>MGSSHHHHHHSGAPGVDVDSSNDRAWRQTQLKVAELLIERQPEVAVGYRLRRHAVWAGITAVPMSGAGN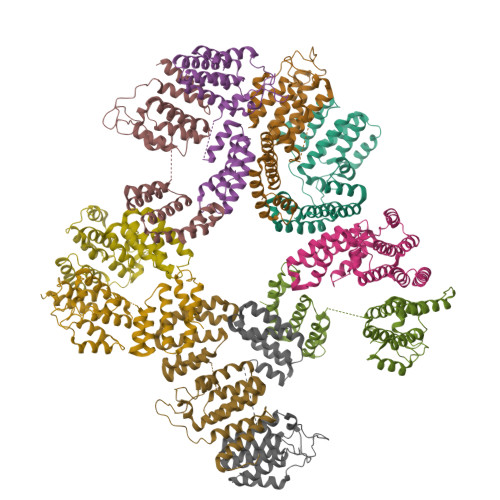KTPLAPMSADMVDEYRAAMNAPDQGLWQRIEQSLTLAPYWFEGHRLSAEVAEKLGFGAVAQAIAEELGTFLQRLPALRELAFSDGSPFLSPECSRWLQPAKGGSAGIGEAGLAEEVAQRHGEQGIAAALALLDERIAQLKEPRDRFHALLVQAELLAQEGMEALARQHYQHLWQEASRLGLSHWEPGLVNRLESLAAPLSK[10x]> DRLTQLQEAMDELLEMFLSAFFWVERHHDLKTFGPNDKIPD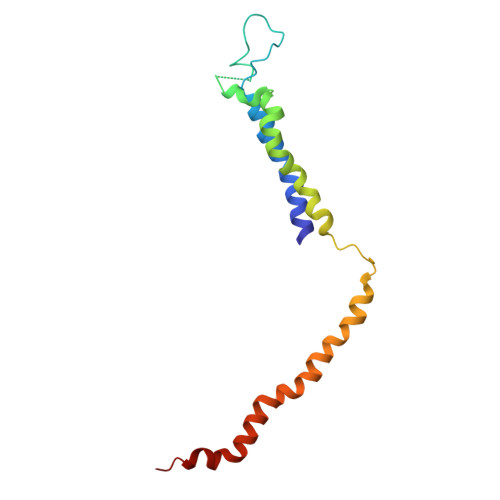LKADQPKEVDTKSPEEYKAGQLQLARDIIVKEQQIEYLISTLPGLDNSEREQIQLLRELEDDLVTAEAQRQEALKERDEVLGKLDALLRGLERP> XRMKQIEDKIEEIE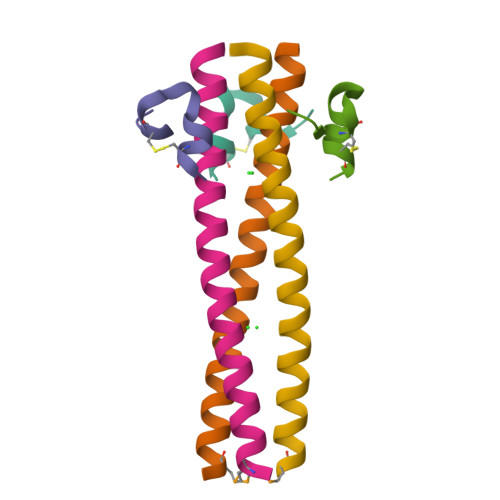SKQKKIENEIARIKKLLQLTVWGIKQLRARILX;> XKGHPCDYPEWQWLCELX>[4x]GPMDPDTNLLKNVILEILSIEPDLYKQSSIVDDPYKLAMSAIRLRATIHELNCCRDLGIIHNTKEISLNMVIDRAIPIHPTFQHIVPDGYTIDR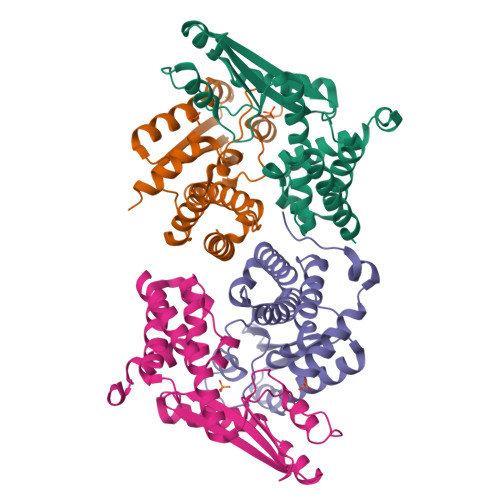ANMTIIVLEASTRSMPSDQKRKITSDKLKYSGVEDHLKHEGWLFNIIVISETKPRNGNVPERLLFELLKLSLSILSYSDKSSQWISEEEYDELKRSLTTYDFKTLTSEFSGTK> MGLSPAFAATAGCRLASPVANSSRFLSLLRLSRPRLNAAAPAAEAAKTLERNVPMKEILQPLWVVEPPNFLRQPVWKQF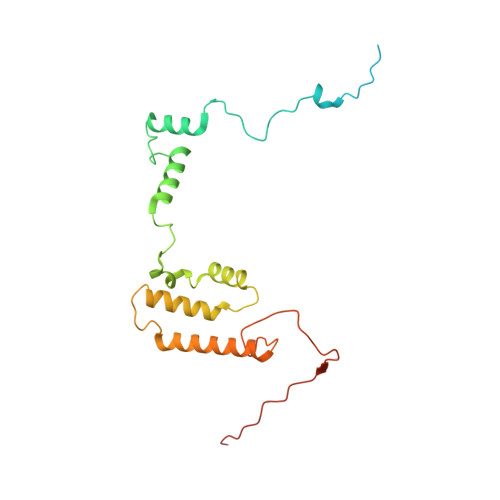WEAQFANRSFFFFGNAWTSAAAFAFFIWWSRVFDPPPKERLDRYWLNSPKFRILSAFHNPGKRPGLKISLMTYEARYCYRGLDHPFTLNEMKDFLFKLREQYLVNKYEGIQFPFVFRQFNRVSTPGTLEVHTSPALQQQPHFHEEAAGHH> GSQSSESLRCNVEPVGRLHIFSGAHGPEKDFPLHLGKNVVGRMPDCSVALPFPSISKQHAEIEILAWDKAPILRDCGSLNGTQILRPPKVLSPGVSHRLRDQELILFADLLCQY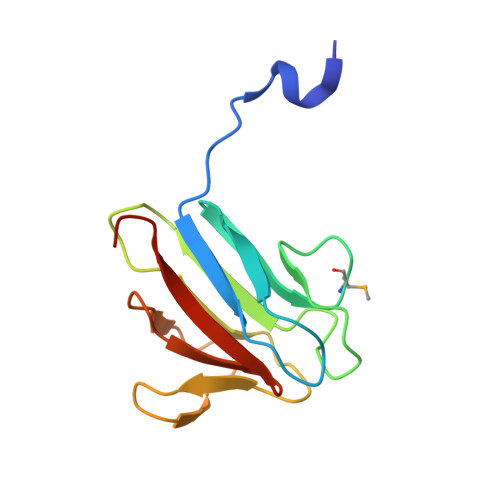HRLDVSLP>AEAGITGTWYNQLGSTFIVTAGADGALTGTYEAAVGNAESRYVLTGRYDSAPATDGSGTALGWTVAWKNNYRNAHSA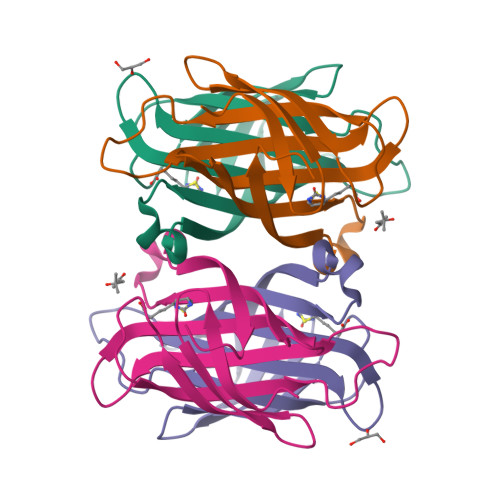TTWSGQYVGGAEARINTQWLLTSGTTEANAWKSTLVGHDTFTKVKPSAAS[2x]>MDFGSLECVVANSAFIAARGSFDASSGPASRDRKYLARLKLPPLSKCEALRESLDLGFEGMCLEQPIGKRLFQQFLRTHEQHGPALQLWKDIEDYD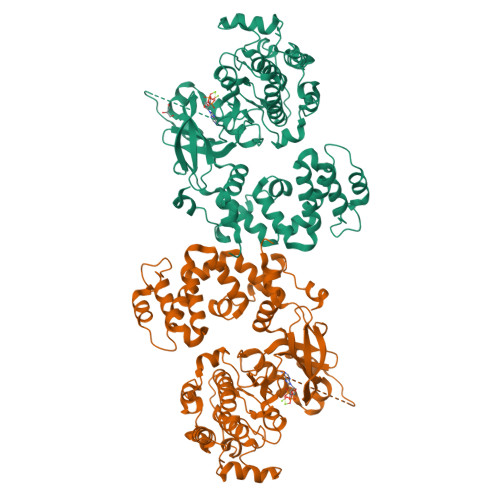TADDALRPQKAQALRAAYLEPQAQLFCSFLDAETVARARAGAGDGLFQPLLRAVLAHLGQAPFQEFLDSLYFLRFLQWKWLEAQPMGEDWFLDFRVLGRGGFGEVFACQMKATGKLYACKKLNKKRLKKRKGYQGAMVEKKILAKVHSRFIVSLAYAFETKTDLCLVMTIMNGGDIRYHIYNVDEDNPGFQEPRAIFYTAQIVSGLEHLHQRNIIYRDLKPENVLLDDDGNVRISDLGLAVELKAGQTKTKGYAGTPGFMAPELLLGEEYDFSVDYFALGVTLYEMIAARGPFRARGEKVENKELKQRVLEQAVTYPDKFSPASKDFCEALLQKDPEKRLGFRDGSCDGLRTHPLFRDISWRQLEAGMLTPPFVPDSRTVYAKCIQDVGAFSTVKGVAFEKADTEFFQEFASGTCPIPWQEEMIETGVFGDLNVWRPDGVDHHHHHH[4x]(2S)-2-AMINO-4-(METHYLSULFANYL)-1-PYRIDIN-2-YLBUTANE-1,1-DIOL | C10 H16 N2 O2 S 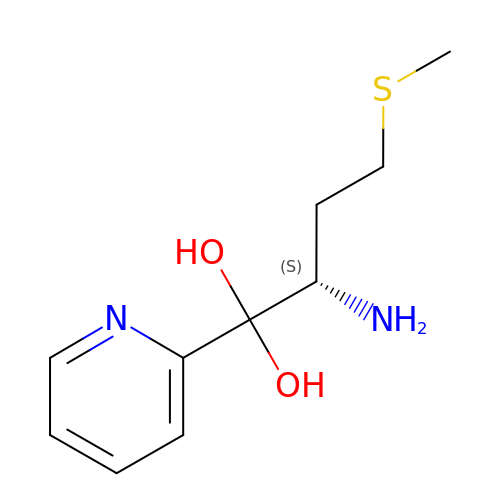| JPZQHIBHGCCNKS-QMMMGPOBSA-N>[4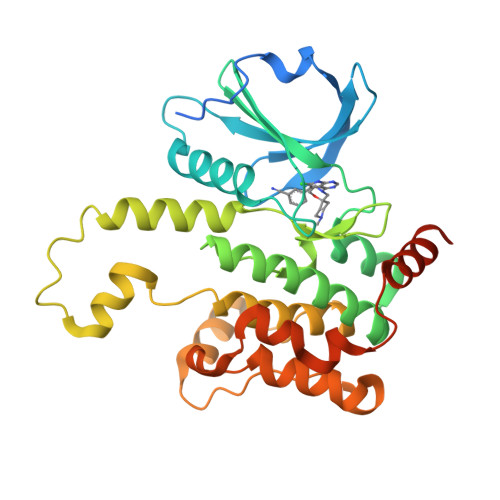x]MASHHHHHHDYDGATTENLYFQGSMDVVDPDIFNRDPRDHYDLLQRLGGGTYGEVFKARDKVSGDLVALKMVKMEPDDDVSTLQKEILILKTCRHANIVAYHGSYLWLQKLWICMEFCGAGSLQDIYQVTGSLSELQISYVCREVLQGLAYLHSQKKIHRDIKGANILINDAGEVRLADFGISAQIGAELARRLEFIGTPYWMAPEVAAVALKGGYNELCDIWSLGITAIELAELQPPLFDVHPLRVLFLMTKSGYQPPRLKEKGKWSAAFHNFIKVTLTKSPKKRPSATKMLSHQLVSQPGLNRGLILDLLDKLKNPGKGPSIGDIEDEE>MSLHACRMKLITAIVKPFTLTDIKDALEQAGVQGMTVTETQGFGQQKGHTEVYRGAEYAVDFVPKVKIEVIISDAQAEEVINIIV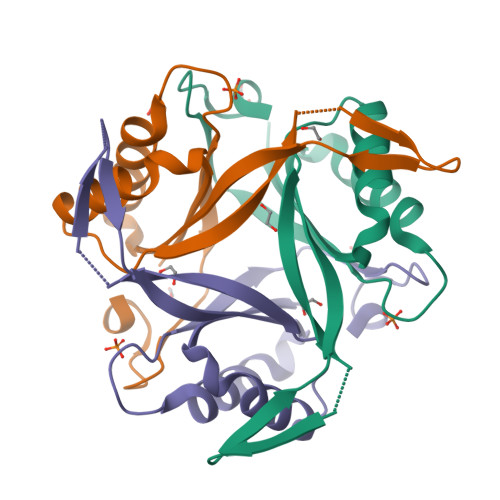ETARTGKVGDGKVWMTNIEELVRVRTGERGEAAL[3x]(R)-2-Aminobutanamide | C4 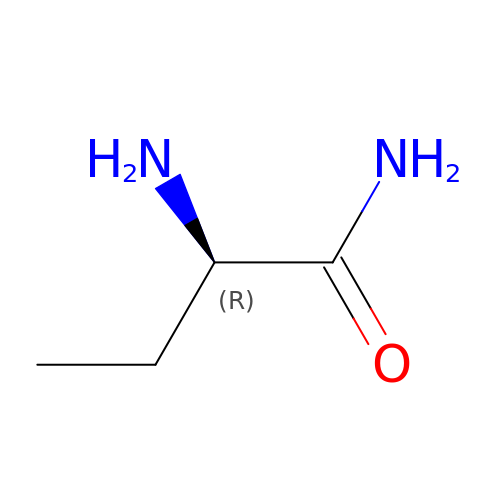H10 N2 O | HNNJFUDLLWOVKZ-GSVOUGTGSA-N> RCSARRANVAALYEFVDGNFLNNKRPAIPGGAWPLESLRRKSLADLQQIWLSLLKERNMLSTIKEHYLRHQEELGAMPAPSRLKMVEESMENVKRVVKERDAEATAEAVRIFKERLAKGIYRYPPGPPPPPGAHDPTSTVKLVLSRRVDEERLRELLGRFNVFEAHKGIVKLTMQLPEDVLTQKRDAEQLWQQYMAERRNVEEYYKWPGSSTGSAESASVYDHTVVELAPGVYSGHRGTSAIESNCVDDSNDGAHGVVQAARLPVPPPKTRPPPPRNPLEHIKYQQRSVLSKAVIQLGYFPNITTTAPRFTKADDVPRPVHPDEIEGPWEVRVTYDAKDGLAYVQSLSLTSIDGAAVLSVEEEFPAAAQPYAAVDPVYQEAVRREMAQEE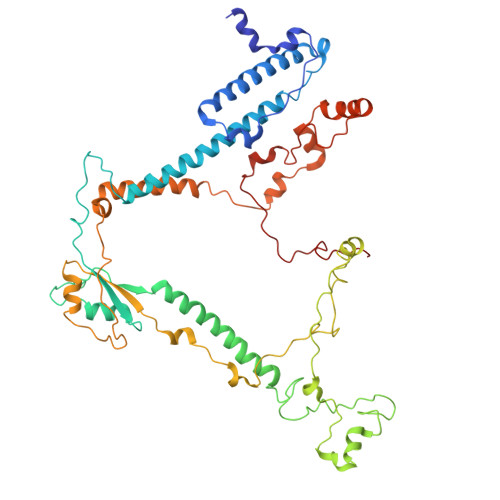TLMKWPNVPKWKYQYDLYTKKHLAQVVQYNYSNVVDYVDREVLLTGRSVWESPIDIDPTCGGMKSVPAHAKKPKRYMTHGLAEVGVTDI> GPMTSQKLVRLPGLIDVHVHLREPGGTHKEDFASGTAAALAGGITMVCAMPNTRPPIIDAPALALAQKLAEAGARCDFALFLGASSENAGTLGTVAGSAAGLKLYLNETYSELRLDSVVQWMEHFETWPSHLPIVAHAEQQTVAAVLMVAQLTQRSVHICHVARKEEILLIKAAKARGLPVTCEVAPHHLFLSHDDLERLGPGKGEVRPELGSRQDVEALWENMAVIDCFASDHAPHTLEEKCGSRPPPGFPGLETMLPLLLTAVSE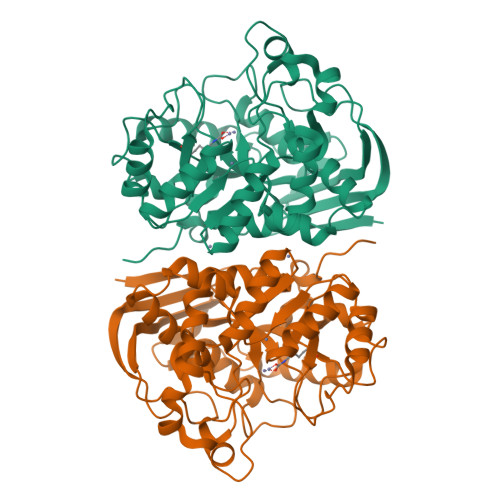GRLSLDDLLQRLHHNPRRIFHLPPQEDTYVEVDLEHEWTIPSHMPFSKAHWTPFEGQKVKGTVRRVVLRGEVAYIDGQVLVPPGYGQDVRKWPQGAVPQLPPSAPATSEMTTTPERPRRGIPGLPD>[2x]MPATDTLSLSASEALARRRSVRAFTDRPVDRALLARIFEIAQRAPSGGNLQPWQATVVTGERWQAVQDAVAARIVMGREGFQPEYDIFPRGLTDPWDSRRFGVGEALYASLGIARDDKAGRIAQFQQNYRGFGAPVMLFLHCSRIMGPPQWADMGMWLQSVMLLLVEHGLASCPQECWAMYGATVRAELGLGDDQILFSGLAIGHADEEAPVNRWPVPRVGLDEVIDWQGFDA

Recently, the nitroreductase NfnB from Sphingopyxis sp. strain HMH exhibited metabolic activity for dinitroaniline herbicides including butralin and pendimethalin, triggering the initial steps of their degradation and detoxification. The homodimer NfnB is a member of the PnbA subgroup of the nitroreductase family. Each monomer displays a central α + β fold for the core domain, with a protruding middle region and an extended C-terminal region. The protruding middle region of Val75–Tyr129 represents a structural extension that is a common feature to members of the PnbA subgroup and functions as an opening wall connecting the coenzyme FMN-binding site to the surface, therefore serving as a substrate binding site.

Next, we determined the crystal structures of the two single mutants, Y88A and Y88F. Their structures were found to be nearly identical to the wildtype NfnB, with RMSD values of 0.38 Å for 428 Cα atoms in Y88A and 0.39 Å for 433 Cα atoms in Y88F. In the Y88F structure, the side chains of Phe88 and Arg100 are well ordered, at positions nearly identical to those of the wildtype NfnB. Compared with the wildtype NfnB, the side chain of Arg100 had been displaced by ∼4 Å toward the side chain of Asp97 near the entrance and was found within a ∼3-Å hydrogen-bonding distance from Asp97. Except for these displacements, no other residues at the entrance exhibited any noticeable conformational changes. Therefore, the possible hydrogen bond between Tyr88 and Arg100 identified in the wildtype NfnB is not crucial for maintaining their side-chain conformations or for NfnB activity. Compared with the wildtype NfnB, the smaller side chain in Y88A and Y88F mutants exhibited a wider opening to the coenzyme FMN. The specific activity of the Y88F mutant against butralin was 97% of the wildtype enzyme, and it showed significantly enhanced activities toward pendimethalin (90%), oryzalin (47%), and isopropalin (14%) compared with the wildtype NfnB for butralin. In particular, Y88F exhibited higher efficiency toward butralin and pendimethalin, with a lower Km value than the wildtype NfnB, but Y88A was more competent than Y88F toward oryzalin and isopropalin, mainly because of its lower Km value. Therefore, even the absence of the side-chain hydroxyl group in the Y88F mutant unexpectedly caused significant changes of many enzymatic properties, without compromising its activity.>MNAIKLYPLKKLEIILEGAHKEFATDLLDRAGVKGYTIVGNLSGKGSHGMYEGHLMFNEDDALIMIIAAVPEELVGPLLEGFQPFFEAHSGVV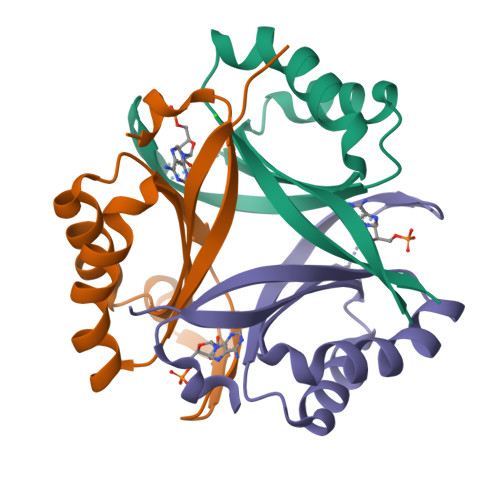FVHDIQVGRPIKFRN[3x]> MQRSPLEKASVVSKLFFSWTRPILRKGYRQRLELSDIYQIPSVDSADNLSEKLEREWDRELASKKNPKLINALRRCFFWRFMFYGIFLYLGEVTKAVQPLLLGRIIASYDPDNKEERSIAIYLGIGLCLLFIVRTLLLHPAIFGLHHIGMQMRIAMFSLIYKKTLKLSSRVLDKISIGQLVSLLSNNLNKFDEGLALAHFVWIAPLQVALLMGLIWELLQASAFCGLGFLIVLALFQAGLGRMMMKYRDQRAGKISERLVITSEMIENIQSVKAYCWEEAMEKMIENLRQTELKLTRKAAYVRYFNSSAFFFSGFFVVFLSVLPYALIKGIILRKIFTTISFCIVLRMAVTRQFPWAVQTWYDSLGAINKIQDFLQKQEYKTLEYNLTTTEVVMENVTAFWEEGFGELFEKAKQNNNNRKTSNGDDSLFFSNFSLLGTPVLKDINFKIERGQLLAVAGSTGAGKTSLLMVIMGELEPSEGKIKHSGRISFCSQFSWIMPGTIKENIIFGVSYDEYRYRSVIKACQLEEDISKFAEKDNIVLGEGGITLSGGQRARISLARAVYKDADLYLLDSPFGYLDVLTEKEIFESCVCKLMANKTRILVTSKMEHLKKADKILILHEGSSYFYGTFSELQNLQPDFSSKLMGCDSFDQFSAERRNSILTETLHRFSLEGDAPVSWTETKKQSFKQTGEFGEKRKNSILNPINSIRKFSIVQKTPLQMNGIEEDSDEPLERRLSLVPDSEQGEAILPXXXXXXXXXXXXXXXXXXXLNLMTHSVNQGQNIHRKTTASTRKVSLAPQANLTELDIYSRRLSQETGLEISEEINEEDLKECFFDDMESIPAVTTWNTYLRYITVHKSLIFVLIWCLVIFLAEVAASLVVLWLLGNTPLQDKGNSTHSRNNSYAVIITSTSSYYVFYIYVGVADTLLAMGFFRGLPLVHTLITVSKILHHKMLHSVLQAPMSTLNTLKAGGILNRFSKDIAILDDLLPLTIFDFIQLLLIVIGAIAVVAVLQPYIFVATVPVIVAFIMLRAYFLQTSQQLKQLESEGRSPIFTHLVTSLKGLWTLRAFGRQPYFETLFHKALNLHTANWFLYLSTLRWFQMRIEMIFVIFFIAVTFISILTTGEGEGRVGIILTLAMNIMSTLQWAVNSSIDVDSLMRSVSRVFKFIDMPTEGKPTKSTKPYKNGQLSKVMIIENSHVKKDDIWPSGGQMTVKDLTAKYTEGGNAILENISFSISPGQRVGLLGRTGSGKSTLLSAFLRLLNTEGEIQIDGVSWDSITLQQWRKAFGVIPQKVFIFSGTFRKNLDPYEQWSDQEIWKVADEVGLRSVIEQFPGKLDFVLVDGGCVLSHGHKQLMCLARSVLSKAKILLLDEPSAHLDPVTYQIIRRTLKQAFADCTVILCEHRIEAMLECQQFLVIEENKVRQYDSIQKLLNERSLFRQAISPSDRVKLFPHRNSSKCKSKPQIAALKEETEEEVQDTRLSNSLEVLFQ

The cystic fibrosis transmembrane conductance regulator (CFTR) is an anion channel that regulates salt and fluid homeostasis across epithelial membranes. CFTR belongs to the ATP-binding cassette transporter family of proteins, but uniquely functions as an ion channel. It consists of two transmembrane domains that form an ion permeation pathway, two cytosolic NBDs that bind and hydrolyse ATP, and a cytosolic regulatory (R) domain that includes several phosphorylation sites. CFTR contains two functionally distinct ATP-binding sites.

In contrast to the case for phosphorylated CFTR, addition of ATP to the dephosphorylated channel caused only a small shift in FRET efficiency, from ≈0.25 to 0.28 ± 0.01. To explore the molecular basis of this shift, we determined the cryo-EM structure of the dephosphorylated wild-type CFTR in the presence of 3 mM ATP to 4.3 Å resolution. Consistent with the smFRET data, the overall CFTR architecture was largely indistinguishable from that of the ATP-free CFTR structure. However, at both NBD1 and NBD2 binding sites, density corresponding to the ATP molecule was clearly evidenced. These data indicate that ATP binding to the dephosphorylated CFTR does not induce any global conformational change. The small shift in FRET efficiency is probably due to local changes that affect either the position and/or dynamics of the sites of labelling. Dephosphorylated CFTR adopts an NBD-separated, auto-inhibited conformation.>MTDNNNYRDVEIRAPRGNKLTAKSWLTEAPLRMLMNNLDPQVAENPKELVVYGGIGRAARNWECYDKIVETLTRLEDDETLLVQSGKPVGVFKTHSNAPRVLIANSNLVPHWANWEHFNELDAKGLAMYGQ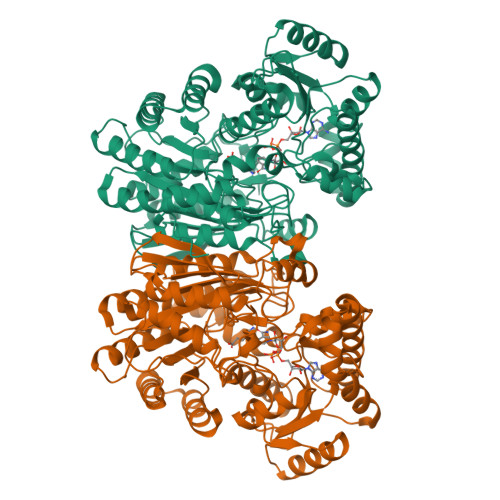MTAGSWIYIGSQGIVQGTYETFVEAGRQHYGGSLKGKWVLTAGLGGMGGAQPLAATLAGACSLNIESQQSRIDFRLETRYVDEQATDLDDALVRIAKYTAEGKAISIALHGNAAEILPELVKRGVRPDMVTDQTSAHDPLNGYLPAGWTWEQYRDRAQTEPAAVVKAAKQSMAVHVQAMLDFQKQGVPTFDYGNNIRQMAKEEGVANAFDFPGFVPAYIRPLFCRGVGPFRWAALSGEAEDIYKTDAKVKELIPDDAHLHRWLDMARERISFQGLPARICWVGLGLRAKLGLAFNEMVRSGELSAPVVIGRDHLDSGSVSSPNAETEAMRDGSDAVSDWPLLNALLNTAGGATWVSLHHGGGVGMGFSQHSGMVIVCDGTDEAAERIARVLTNDPGTGVMRHADAGYDIAIDCAKEQGLDLPMITG[2x]> MRGQGRKESLSDSRDLDGSYDQLTGHPPGPTKKALKQRFLKLLPCCGPQALPSVSETLAAPASLRPHRPRLLDPDSVDDEFELSTVCHRPEGLEQLQEQTKFTRKELQVLYRGFKNECPSGIVNEENFKQIYSQFFPQGDSSTYATFLFNAFDTNHDGSVSFEDFVAGLSVILRGTVDDRLNWAFNLYDLNKDGCITKEEMLDIMKSIYDMMGKYTYP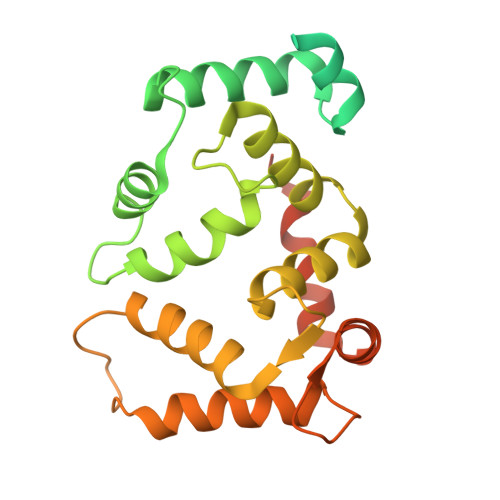ALREEAPREHVESFFQKMDRNKDGVVTIEEFIESCQKDENIMRSMQLFDNVILEGGSSGGHHHHHHHH>KIIYPN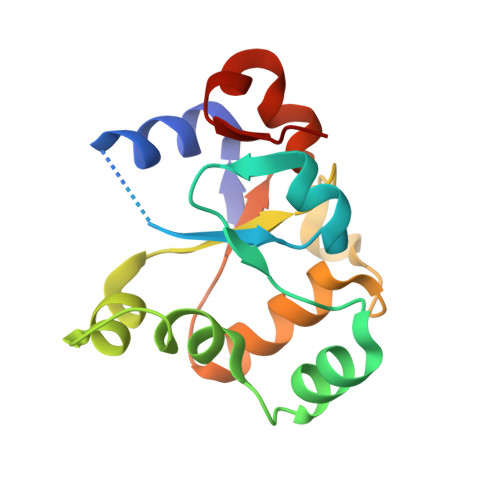DLAKKMTKCSKSHLPSQGPVIIDCRPFMEYNKSHIQGAVHINCADKISRRRLQQGKITVLDLISCREGKDSFKRIFSKEIIVYDENTNEPSRVMPSQPLHIVLESLKREGKEPLVLKGGLSSFKQNHENLCDNSKE[2x]> MKELMRNVYLLDDTLVTKSKYGSHYGEKVFDGYREWVPWRSKLAAMILKGHRLKLRGDERVLYLGAASGTTVSHLADIVDEGIIYAVEYSAKPFEKLLELVRERNNIIPLLFDASKPWKYSGIVEKVDLIYQDIAQKNQIEILKANAEFFLKEKGEVVIMVKARSIDSTAEPEEVFKSVLKEMEGDFKIVKHGSLMPYHRDHIFIHAYRF;> LRYNLWFGVYDGKEIKLSENFEESFLKAENPSPLPFNVSEVGAKALGKDYYRILRKTALAVSEKMVEKELRREDRYVVALVKALEEIDESINMLNEKLEDIRAV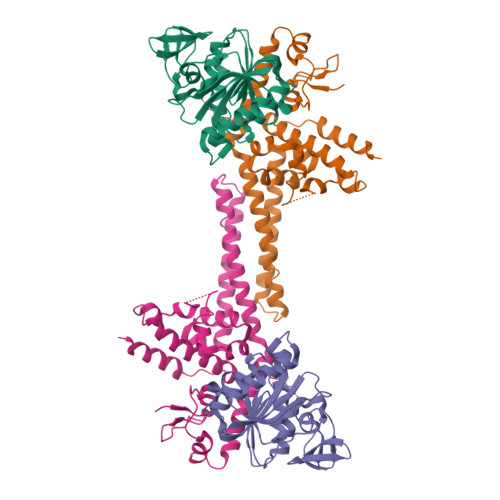KESEITEKFEKKIRELRELRRDVEREIEEVMEKIAPNMTELVGAKVAAKLLERAGSMERLVRLPASKIQVIGAEKSLYKAFARMKKGKKAKIPKHGIIFLHPFIRTLPKAKRGKMARFLAAKLAIAAKIDYFRGEIDESLYESIRRRYEELRRK> MRT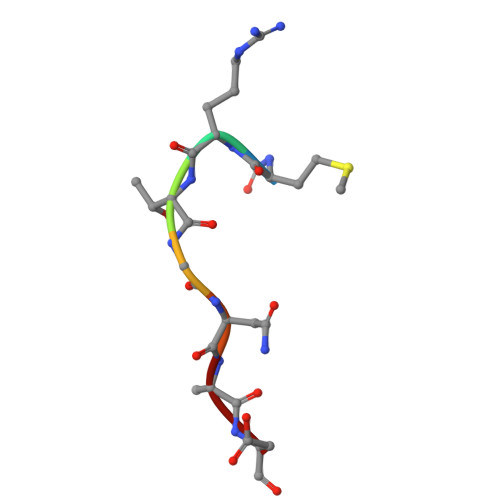GNAD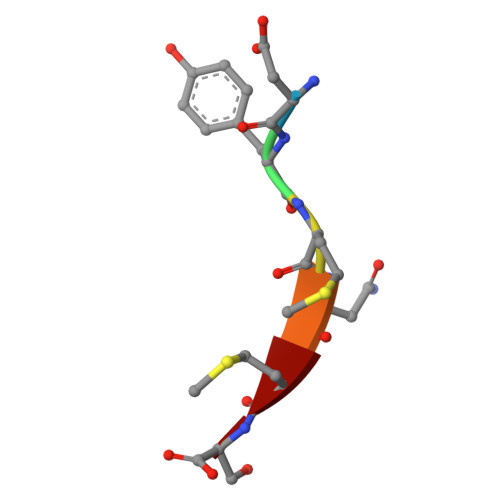> DYMNMS>[2x]REVLTGGHSVSAPQ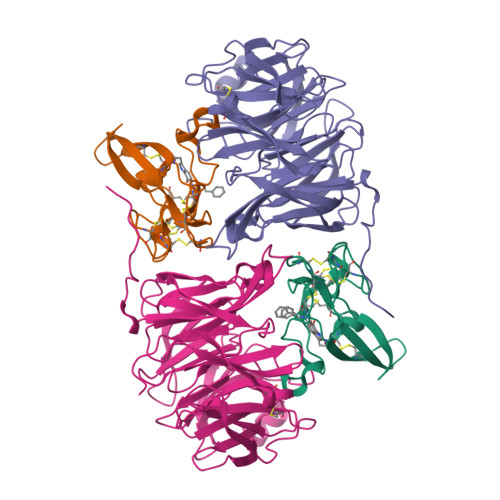ENRIYVMDSVFMHLTESRVHVYDYTNGKFLGMVPTAFNGHVQVSNDGKKIYTMTTYHERITRGKRSDVVEVWDADKLTFEKEISLPPKRVQGLNYDGLFRQTTDGKFIVLQNASPATSIGIVDVAKGDYVEDVTAAAGCWSVIPQPNRPRSFMTICGDGGLLTINLGEDGKVASQSRSKQMFSVADDPIFIAPALDKDKAHFVSYYGNVYSADFSGDEVKVDGPWSLLNDEDKAKNWVPGGYNLVGLHRASGRMYVFMHPDGKEGTHKFPAAEIWVMDTKTKQRVARIPGRDALSMTIDQQRNLMLTLDGGNVNVYDISQPEPKLLRTIEGAAEASLQVQFHPVGGT;>[2x]AGGGGSSSGADHISLNPDLANEDEVNSCDYWRHCAVDGFLCSCCGGTTTTCPPGSTPSPISWIGTCHNPHDGKDYLISYHDCCGKTACGRCQCNTQTRERPGYEFFLHNDVNWCMANENSTFHCTTSVLVGLAKN> GAPSLINSEDNPAF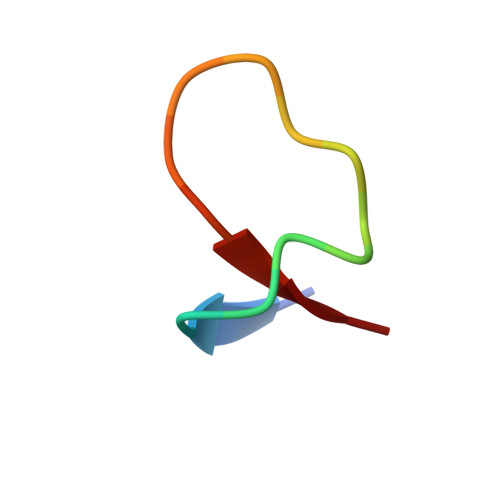PQRV The outer membrane cytochrome F (OmcF) is one of these proteins. OmcF is a 104 amino acids protein with a predicted small lipid anchor at the N-terminus formed by the first 19 residues, a soluble domain consisting of residues 20–104 and a low-spin c-type heme group with axial His-Met coordination. The structure of OmcF showed high similarity to those of cytochromes c6 from photosynthetic algae and cyanobacteria, particularly from Scenedesmus obliquus and Monoraphidium braunii. The cytochrome OmcF from the bacterium G. sulfurreducens showed an important pH modulation of the heme reduction potential (redox-Bohr effect) in physiological range for G. sulfurreducens cellular growth.

The protonatable site of the imidazole ring of histidine 47 (His47) has been hypothesized as the redox-Bohr center based: (i) on the typical pKa value for a histidine side chain and (ii) on its spatial location near the heme in the structure of OmcF (Dantas et al., 2017). To test this hypothesis, in the present work, we used site-directed mutagenesis to replace the His47 by isoleucine (OmcFH47I) and phenylalanine (OmcFH47F) residues. In both cases, the side chain of the substituting residues is not protonatable and, therefore, will permit the evaluation of the contribution of His47 to the observed redox-Bohr effect. In addition, the crystal structure of the OmcFH47I mutant was determined. The crystal structure of OmcFH47I mutant determined at a high resolution also showed that the mutation did not affect the structure. The global folding of the mutants was assessed by NMR spectroscopy and the comparison of the polypeptide and heme NMR signals showed that both the mutants were properly folded and that only local conformational changes were observed in the vicinity of the mutated residue regions. Electrochemical cyclic voltammetry studies carried out for both the mutants, within the physiological pH range, showed that the redox potential values and the redox-Bohr effect were smaller compared to the wild-type cytochrome. This unequivocally confirms the role of His47 in the pH modulation of the OmcF heme redox potential and electron/proton transfer mechanisms. However, the redox-Bohr effect was not fully abolished in the mutants (approximately 30% less in the mutants) suggesting the existence of another redox-Bohr center in OmcF, which was attributed to the heme propionate P13. Therefore, these two acid–base groups with pKa in the physiological range (heme propionate P13 and His47) contribute to the overall observed redox-Bohr effect.

> AGAGGGELFATHCAGCHPQGGNTVIPEKTLARARREANGIRTVRDVAAYIRNPGPGMPAFGEAMIPPADALKIGEYVVASFP Orthologous proteins to ependymin called ependymin-related proteins (EPDRs) have been found to exist in various tissues from sea urchins to humans, yet their functional role remains to be revealed. All of the EPDR1s fold into a dimer using a monomeric subunit that is mostly made up of two stacking antiparallel β-sheets with a curvature on one side, resulting in the formation of a deep hydrophobic pocket. All six of the cysteine residues in the monomeric subunit participate in the formation of three intramolecular disulfide bonds. The EPDR1 fold is very similar to the folds of bacterial VioE and LolA/LolB, which also use a similar hydrophobic pocket for their respective functions as a hydrophobic substrate-binding enzyme and a lipoprotein carrier, respectively.

The frog EPDR1 structure was determined first by direct phasing using single-wavelength anomalous diffraction (SAD) from a xenon-derivatized crystal, and the structure was subsequently used as a search model to determine the mouse and human EPDR1 structures by molecular replacement. Only one molecule of frog EPDR1 was found in the asymmetric unit of the crystal of frog EPDR1. All other contacts bury a BSA of less than 500 Å2, with no conservation in other crystal forms. In the frog EPDR1 crystal with only one monomeric subunit in the asymmetric unit, the same dimeric interface was formed between the crystallographic symmetry mates [BSA of ∼2300 Å2 per subunit; Supplementary Fig. S4(c)]. Also, the β8–β9 and β10–β11 loops in frog EPDR1 diverge significantly in comparison to those from human and mouse. In particular, the displacement of the β10–β11 loop towards β1 in frog EPDR1 confers an altered conformation of the shortened β10 and β11. Lastly, α2 at the C-terminus of the human and mouse EPDR1s extends into a loop in frog EPDR1. Although we do not have direct evidence, we have modeled this metal as a Ca2+ ion, which is likely to originate from the 0.2 M calcium acetate condition that was only present in the crystallization reservoir used to obtain the frog EPDR1 crystal. The Ca2+ ion is octahedrally coordinated by four water molecules, the side-chain O atom of Asp121 and the main-chain O atom of Pro122. The four water molecules coordinated to the Ca2+ ion are further stabilized and arranged in place by hydrogen-bonding interactions with the nearby residues Asp124, Glu175 and Tyr177 [Fig. 3(c)].

> ADPHHHHHHHHPVTPCEAPLQWEGRIVLYDHNTGKNTRATVTYDAILQRIRILEEKKSFVPCKRFFEYIFLYQEAVMFQIEQVTKICSKNTLTEPWDPYDIPENSTYEDQYYIGGPGDQIPVQEWSDRKPARKYETWVGVYTVKDCYPVQETYTKNDSMTTSTRFFDIKLGISDPSVFNPPSTCEAAQPLLMSGDC> VKWYYKTITFLPELCNNESLAAKCLRVLHGFNYQYETRNIGVSFPLWCDATVGKKISFVSKNKIELDLLLKQHYFVQMEQLQYFHISNTVLVPEDCTYVSFRRCQSIDKLTAAGLARKI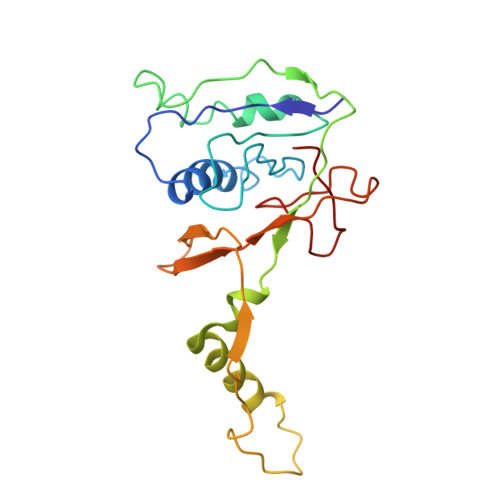RRLEKRALSRGEQFDPSSFAQKEHTAIAHYHSLGESSKQTNRNFRLNIRMLSEQPREGNSIFSSYGLSNSENSFQPVPLI>[6x]MDSFNPTTKTQAALTAALQAASTAGNPEIRPAHLLMALLTQNDGIAAPLLEAVGVEPATVRAETQRLLDRLPQATGASTQPQLSRESLAAITTAQQLATELDDEYVSTEHVMVGLATGDSDVAKLLTGHGASPQALREAFVKVRGSARVTSPEPEATYQALQKYSTDLTARAREGKLDPVIGRDNEIRRVVQVLSRRTKNNPVLIGEPGVGKTAIVEGLAQRIVAGDVPESLRDKTIVALDLGSMVAGSKYRGEFEERLKAVLDDIKNSAGQIITFIDELHTIVGAGATGEGAMDAGNMIKPMLARGELRLVGATTLDEYRKHIEKDAALERRFQQVYVGEPSVEDTIGILRGLKDRYEVHHGVRITDSALVAAATLSDRYITARFLPDKAIDLVDEAASRLRMEIDSRPVEIDEVERLVRRLEIEEMALSKEEDEASAERLAKLRSELADQKEKLAELTTR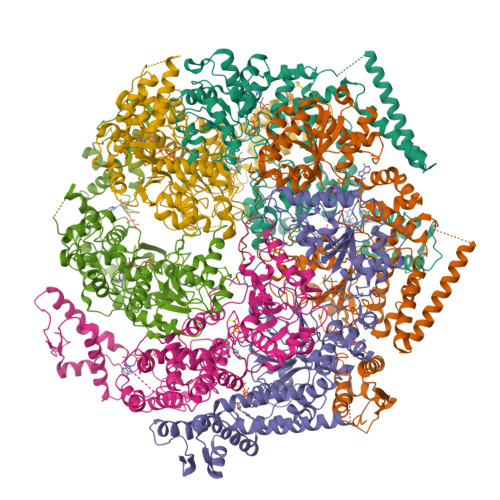WQNEKNAIEIVRDLKEQLEALRGESERAERDGDLAKAAELRYGRIPEVEKKLDAALPQAQAREQVMLKEEVGPDDIADVVSAWTGIPAGRLLEGETAKLLRMEDELGKRVIGQKAAVTAVSDAVRRSRAGVSDPNRPTGAFMFLGPTGVGKTELAKALADFLFDDERAMVRIDMSEYGEKHTVARLIGAPPGYVGYEAGGQLTEAVRRRPYTVVLFDEIEKAHPDVFDVLLQVLDEGRLTDGHGRTVDFRNTILILTSNLGSGGSAEQVLAAVRATFKPEFINRLDDVLIFEGLNPEELVRIVDIQLAQLGKRLAQRRLQLQVSLPAKRWLAQRGFDPVYGARPLRRLVQQAIGDQLAKMLLAGQVHDGDTVPVNVSPDADSLILG;> AAAAAAAAAAAAAAAAAAAAAAAAAA[(2~{R},3~{S},4~{R},5~{R})-5-[6-(ethylamino)purin-9-yl]-3,4-bis(oxidanyl)oxolan-2-yl]methyl 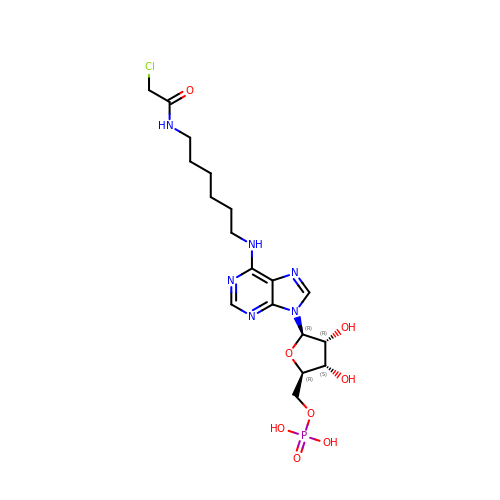dihydrogen phosphate | C18 H28 Cl N6 O8 P | QFONDZUXFQHEPG-XKLVTHTNSA-N> HQRKVVSWIDVYTRATCQPREVVVPLTVELMGTVAKQLVPSCVTVQRCG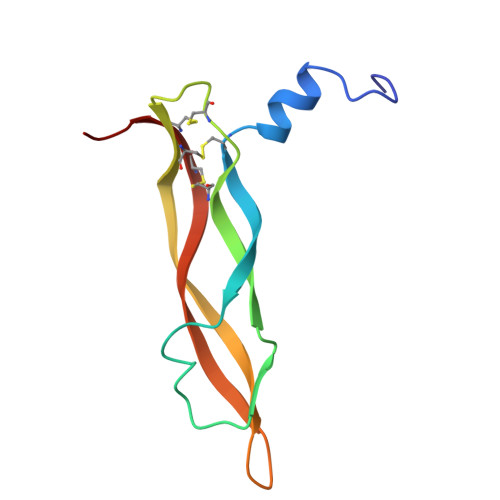GCCPDDGLECVPTGQHQVRMQILMIRYPSSQLGEMSLEEHSQCECRPKKK(2E)-3-(3-fluoro-4-hydroxyphenyl)-2-{[(Z)-{3-hydroxy-2-methyl-5-[(phosphonooxy)methyl]pyridin-4(1H)-ylidene}methyl]imino}propanoic acid | C17 H18 F N2 O8 P | 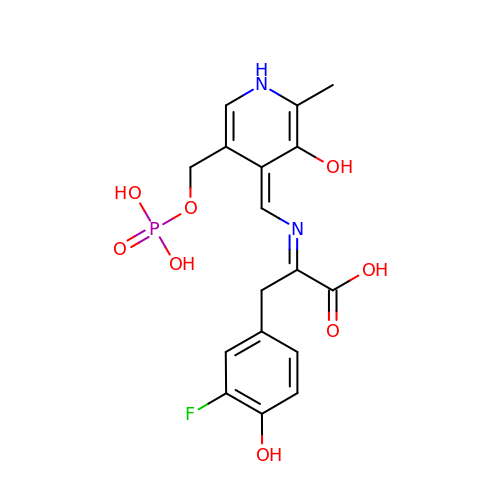AWZHPOMIAYWMIB-ALAGMBGBSA-N>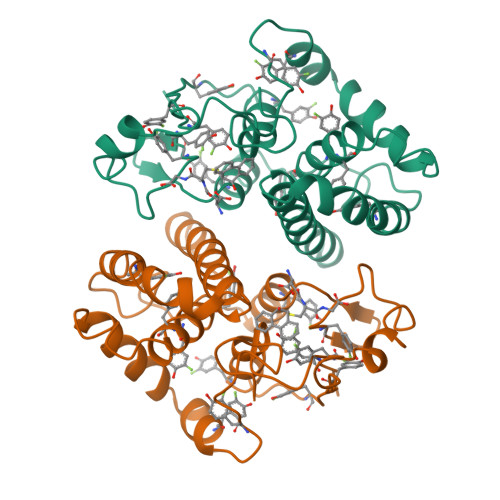PMILGYWNVRGLTHPIRLLLEYTDSSYEEKRYAMGDAPDYDRSQWLNEKFKLGLDFPNLPYLIDGSRKITQSNAIMRYLARKHHLCGETEEERIRADIVENQVMDNRMQLIMLCYNPDFEKQKPEFLKTIPEKMKLYSEFLGKRPWFAGDKVTYVDFLAYDILDQYHIFEPKCLDAFPNLKDFLARFEGLKKISAYMKSSRYLSTPIFSKLAQWSNK[2x]>MDYKDDDDKEEGFRDRAAFIRGAKDIAKEVKKHAAKKVVKGLDRVQDEYSRRSYSRFEEEDDDDDFPAPSDGYYRGEGTQDEEEGGASSDATEGHDEDDEIYEGEYQGIPRAESGGKGERMADGAPLAGVRGGLSDGEGPPGGRGEAQRRKEREELAQQYEAILRECGHGRFQWTLYFVLGLALMADGVEVFVVGFVLPSAEKDMCLSDSNKGMLGLIVYLGMMVGAFLWGGLADRLGRRQCLLISLSVNSVFAFFSSFVQGYGTFLFCRLLSGVGIGGSIPIVFSYFSEFLAQEKRGEHLSWLCMFWMIGGVYAAAMAWAIIPHYGWSFQMGSAYQFHSWRVFVLVCAFPSVFAIGALTTQPESPRFFLENGKHDEAWMVLKQVHDTNMRAKGHPERVFSVTHIKTIHQEDELIEIQSDTGTWYQRWGVRALSLGGQVWGNFLSCFGPEYRRITLMMMGVWFTMSFSYYGLTVWFPDMIRHLQAVDYASRTKVFPGERVEHVTFNFTLENQIHRGGQYFNDKFIGLRLKSVSFEDSLFEECYFEDVTSSNTFFRNCTFINTVFYNTDLFEYKFVNSRLINSTFLHNKEGCPLDVTGTGEGAYMVYFVSFLGTLAVLPGNIVSALLMDKIGRLRMLAGSSVMSCVSCFFLSFGNSESAMIALLCLFGGVSIASWNALDVLTVELYPSDKRTTAFGFLNALCKLAAVLGISIFTSFVGITKAAPILFASAALALGSSLAL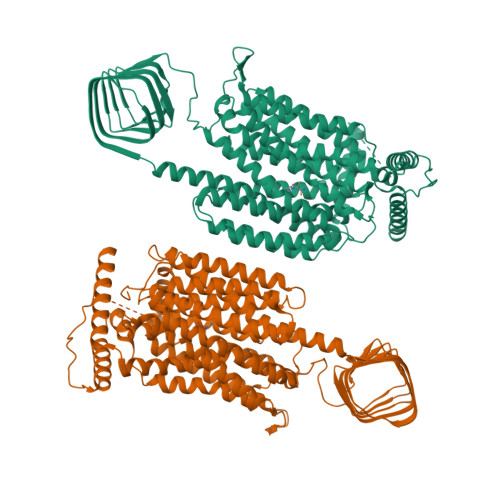KLPETRGQVLQ[2x]> GPMALDICVKVAVGAPDVLGDCPFSQRVLLTLEEKKLPYKTHLINVSDKPQWFLDISPEGKVPVVKLDGKWVADSDVIVGLLEEKYPEPSLKTPPEFASVGSKIFGAFVTFLKSKDANDGSEKALVDELEALENH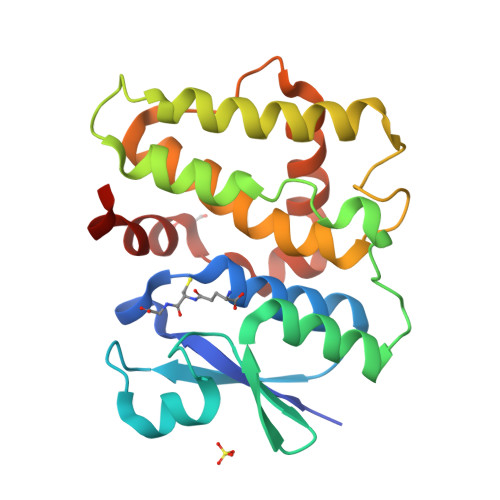LKTHSGPFVAGEKITAVDLSLAPKLYHLEVALGHYKNWSVPESLTSVRNYAKALFSRESFENTKAKKEIVVAGWESKVNA> MFFSRLSLSALKAAPAREALPGLLSRQSFSSAGFSQFSSQKFFFSPSRNFSQSPLFQKHTPVHCNQRIASALVPTQQPAMTRQNPYAMQVGARYDAGVASLSAAIALMSVGGVAQGIGS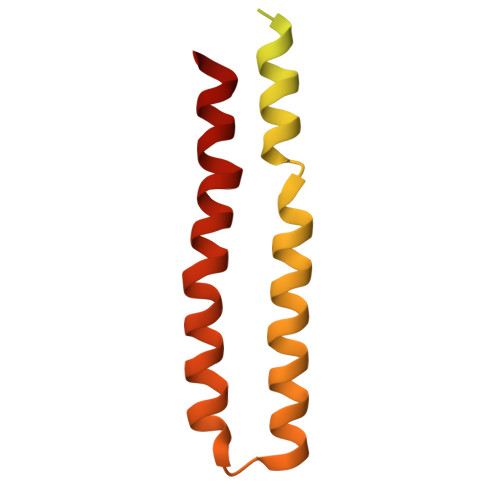LFAALVSGTARNPSIKEDLFTYTLIGMGFLEFLGIICVLMSAVLLYS>MNYLNNIRIENPLTICYTNDVVKNFTANGLLSIGASPAMSEAPEEAEEFYKVAQALLINIGTLTAQNEQDIIAIAQTANEAGLPIVFDPVAVGASTYRKQFCKLLLKSAKVSVIKGNASEILALIDDTATMKGTDSDANLDAVTIAKKAYAIYKTAIVITGKEDVIVQGDKAIVLANGSPLLARVTGAGCLLGGIIAGFLFRETEPDIEALIEAVSVFNIAAEVAAENENCGGPGTFSPLLLDTLYHLNETTYQQ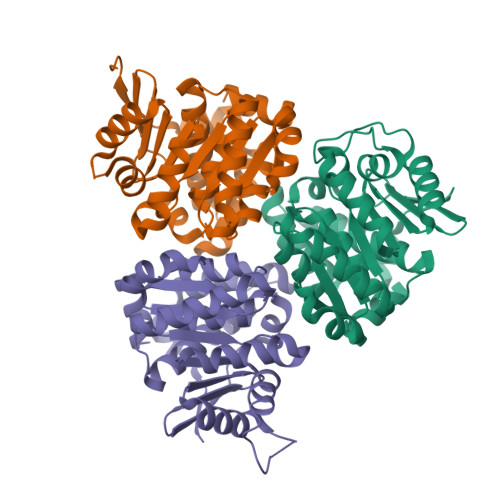RIRIQEVEENLYFQSGHHHHHH[6x]Sirtuins are an evolutionarily conserved family of NAD+-dependent protein deacetylases, with seven isoforms, Sirt1-7, in mammals. Sirt1 features the conserved Sirtuin catalytic core of ~270 amino acids, which consists of a large NAD+-binding Rossmann fold subdomain and a small, structurally more variable Zn2+-binding subdomain. The binding site for the acetyllysine-containing protein substrate is a cleft between these two subdomains, which undergo a closure movement upon binding of substrate and/or NAD+ cosubstrate. A biochemical characterization of the interaction including binding and stability assays, NMR spectroscopy, mass spectrometry, and a crystal structure of Sirtuin/AROS peptide complex reveal that AROS acts as a competitive inhibitor, through binding to the Sirt1 substrate peptide site.

We can conclude, however, that the key elements for Sirt1 inhibition by AROS are present in the generic Sirtuin catalytic core that is shared by all isoforms, and that we can thus exploit other isoforms as model systems for structural and mechanistic studies on its interaction with AROS. We solved a crystal structure of Sirt3 in complex with a peptide AROS 62-71 at 3.27 Å resolution. The structure was refined to Rcryst/Rfree values of 20.2/26.1%. The electron density revealed the Arg-Lys-Arg motif of the peptide ligand to be bound to the substrate binding groove, with AROS Lys65 in the active site pocket for the substrate acetyl-lysine, packed between His248 and Phe180/294. Arg66 is stacked upon Phe294, and Arg64 interacts with the mainchain oxygen of Leu298. Beyond these three AROS residues, the ligand is not well defined by electron density and appears to be flexible, without major contact with the Sirtuin. Comparing the complex to other Sirtuin/peptide complexes (Sirt3/ACS2, Sirt5/IDH2, Sirt1/p53) confirms that both types of ligands share the more closed Sirtuin conformation generally observed for Sirtuin/substrate complexes and the high conservation of residues interacting with the visible core motif of the respective ligand. The comparison indicates only subtle differences in the local Sirtuin conformation (small rotations of Sirt3 His248 and Phe294), likely caused by the Lys acylation of substrate peptides. The only significant difference between the AROS motif and a substrate appears to be the side-chain position of AROS-Arg66, which appears to occupy the pocket normally accommodating the backbone of one or two additional defined residues and thereby supports AROS binding and its ability to compete with physiological substrates.

>[6x]MAFWGWRAAAALRLWGRVVERVEAGGGVGPFQACGCRLVLGGRDDVSAGLRGSHGARGEPLDPARPLQRPPRPEVPRAFRRQPRAAAPSFFFSSIKGGRRSISFSVGASSVVGSGGSSDKGKLSLQDVAELIRARACQRVVVMVGAGISTPSGIPDFRSPGSGLYSNLQQYDLPYPEAIFELPFFFHNPKPFFTLAKELYPGNYKPNVTHYFLRLLHDKGLLLRLYTQNIDGLERVSGIPASKLVEAHGTFASATCTVCQRPFPGEDIRADVMADRVPRCPVCTGVVKPDIVFFGEPLPQRFLLHVVDFPMADLLLILGTSLEVEPFASLTEAVRSSVPRLLINRDLVGPLAWHPRSRDVAQLGDVVHGVESLVELLGWTEEMRDLVQRETGKLDGPDK;>MSAALLRRGLELLAASEAPRDPPGQAKPRGAPVKRPRKTKAIQAQKLRNSAKGKVPKSALDEYRKRECRDHLRVNLKFLTRTRSTVAESVSQQILRQNRGRKACDRPVAKTKKKKAEGTVFTEEDFQKFQQEYFGS[6x]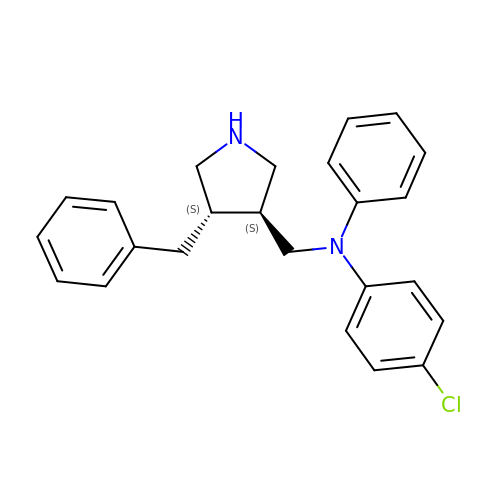N-{[(3S,4S)-4-benzylpyrrolidin-3-yl]methyl}-4-chloro-N-phenylaniline | C24 H25 Cl N2 | FCWGSUKXROLTNW-RTWAWAEBSA-N> MNELSKKY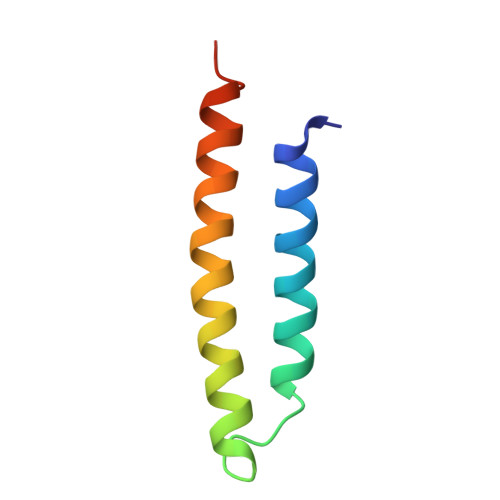LAKVKERHELKEFNNSISAQDNYAKWTKNNRKLDSLDKEINNLKDEIQSENHHHHHH>[2x]MKNELIKRIGIFVCLLIAVNCLSAGNFPVEMRINPSTGAIS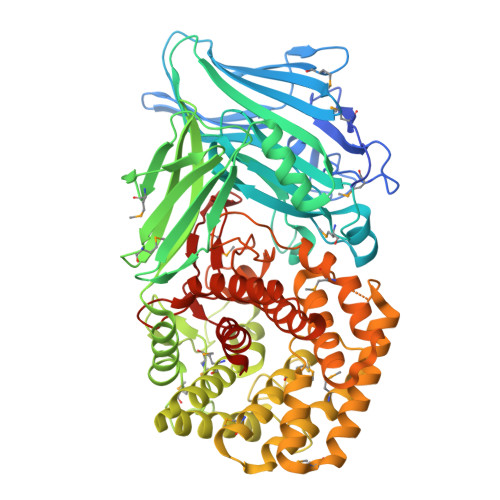ELTLKGDNRSMNWVVKTDGTQYPWVKDNYGWGLGYFTVVKGRETVKREWRIPVEISPDGMKVLYREGDIRILIKREIKQGDLVEEYSFTNEGEEPVSLYDVAVYTPFNDNYPDAQQCINSRAHTHIWKGGSAAYVNAIRMGDFTPHLGLVVTDGAIRNYEIWERGRKKANSQTRGIIALDLPDLLLKPGESYSLEWHVFAHNGNDDFRHKLLEKGSVLVSCNKYVFEKGEKARVECRSLEPLEACTAKMNGVPVPVKQEGNLCFVEVPMEQAGEVRFDFYYNGNKQTHADCLVISNTADLIRKRVDFIRTRQQMNNPSDLRDGAYMVYDNEGDSIYLNDTPNCNPVDRDEGAERLGMGVLLVKQYLLTKDPELKQSLLRYADFVRRKLQTDNYVTYSSVDQKNRNRGYNYMWVAELYFQMYKVTGDKQFVTDGYKTLKSMFQQFGYGFYAIGIPVRLGLQSLKEAGMKKEYTDLRNDFIKTGDVFVKNGLNYPAHEVNYEQSIVAPAIQFLAQLYLETGSQKYLDEVKRQMPVLEAFNGFQPSYHLNEVAIRHWDGHWFGKRELFGDTFPHYWSTITGAVYYYYALCTGDSSYQKRAENVVRNNLCLFFEDGKASCAYMYPYKIDGVKAEFYDPYANDQDWALVYYLLVNRGL>[4x]QDNCTCPTNKMTVCSPDGPGGRCQCRALGSGMAVDCSTLTSKCLLLKARMSAPKNARTLVRPSEHALVDNDGLYDPDCDPEGRFKARQCQQTSVCWCVNSVGVRRTDKGDLSLRCDELVRTH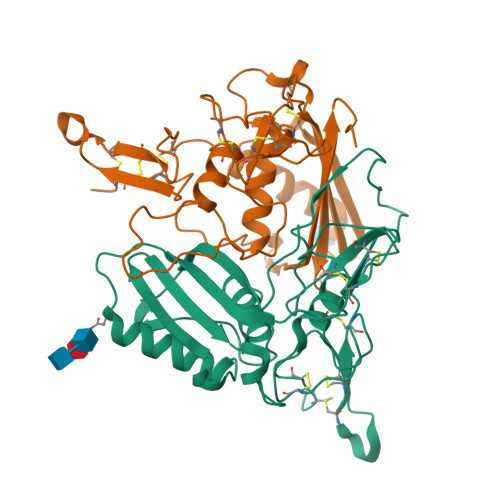HILIDLRHRPTAGAFNHSDLDAELRRLFRERYRLHPKFVAAVHYEQPTIQIELRQQTSQKAAGDVDIGDAAYYFERDIKGESLFQGRGGLDLRVRGEPLQVERTLIYYLDEIPPKFSMKRLTHHHHHH>RRRSGSLVYQKRRRRLLPFVSSEDPAQRLKQMGTLASALTELQMEFSDDLTYSSGMAPRSANQARFEEGGMQVLTKEDIETLEQCRAMCKRGDCPPLLVVFDSREGFTVEADGQIKDMTFIAEYTGDVDYIRNREHDDCDSMMTLLLAKDPSSSLVICPDKRGNIARFISGINNHTLDAKKKQNCKCVRYSVNGECRVFLVATRDIAKGERLYYDYNGYEHEYPTQHFV[2x]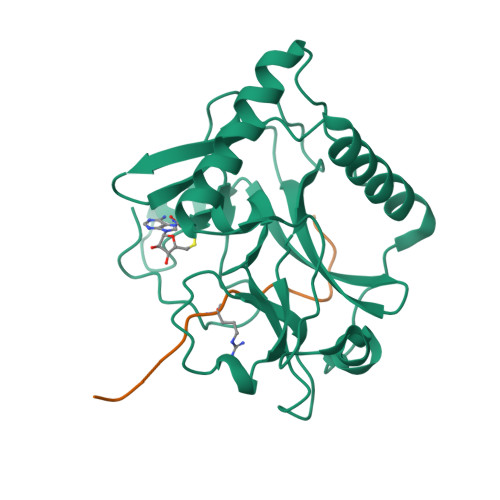;>QLATKAARKSAPATGGVK[2x]In the recently identified TreS-Mak-GlgE-GlgB pathway maltose is produced by TreS, phosphorylated by Mak into maltose-1-phosphate (M1P), and then used for glycogen elongation by the maltosyltransferase GlgE56. The structure of MakMvan, which shares 59% amino acid sequence identity with MakMtb, revealed a typical bilobal eukaryotic protein kinase-like (ELK) fold, conserving the main structural motifs required for the phosphotransfer reaction. Strikingly, MakMvan displays a novel N-terminal domain, unique to maltokinases and conserved in the bifunctional TreS-Mak proteins, and without sequence similarity to other known proteins. MakMvan used ATP as the favourite phosphate donor, being strictly dependent on divalent cations, with a clear preference for Mg2+.

MakMvan crystallized in the orthorhombic space group P2221 and diffracted to 1.47 Å resolution. The protein displays an elongated concave-shaped structure that can be divided into two half-lobes with a central narrow acidic channel (~9 Å-wide and 30 Å-long), delineated by a positively charged surface patch on the N-terminal lobe and a negatively charged region on the C-terminal lobe, and displaying basic character at its exit site. The N-terminal lobe can be divided into two subdomains: a cap N-terminal subdomain comprising the first 88 amino acid residues (blue) and an intermediate subdomain composed of an anti-parallel β-sheet flanked by two helices (green). The C-terminal lobe is mostly α-helical (dark red). Analysis of the B-factor distribution reveals that the cap subdomain has the highest values for the atomic temperature factors and the C-terminal domain the lowest, suggesting that the N-terminal lobe, in particular the cap region, is more dynamic. As observed in related ELKs, His303 (HGD motif) stacks with Phe323 of the magnesium-coordinating DFE motif in the structure of free MakMvan. In the structure of free MakMvan the largest pocket identified (pocket 1) is located to the left of the exposed catalytic cleft and delineated by strictly conserved residues within the C-terminal lobe (dark blue spheres). Pocket 1 is close to the active site HGD motif and includes Asp305, topologically equivalent to the catalytic base in analogous enzymes (e.g. MTR32), and globally coincident with the substrate-binding region in structurally related ELKs. However, considering the overall higher conservation of pocket 1 in MakMvan three-dimensional structure, which is topologically equivalent to the substrate-binding region in other ELKs, this cavity most likely represents the maltose-binding site.

> MTLAFGDWIVHRRWYAGRSRELVSAEPAVVTPLRDDLDHILLDVTYTDGTVERYQLVVRWADSPVAGFGEAATIGTALGPQGERIAYDALFDPDAARHLLRLVDASATVADLRFTREPGATLPLYAPPKVSSAEQSNTSVIFGKDAMLKVFRRVTPGINPDIELNRVLAQAGNRHVARLLGSFETSWAGPGTDRCALGMVTAFAANSAEGWDMATASAREMFADVVGSDFADESYRLGNAVASVHATLAEALGTSTEPFPVDTVLARLQSAARSAPELAGRAAAVEERYRRLDGRAITVQRVHGDLHLGQVLRTPDDWLLIDFEGEPGQPLDERRRPDSPLRDVAGVLRSFEYAAYQKLVELAPEQDADGRLADRARNWVDRNSAAFCAGYAAVAGDDPRRDGDVLAAYELDKAVYEAAYEARFRPSWLPIPMRSIDRILGKLAAALEHHHHHH2-methylpropyl N-[(2S)-1-oxidanylidene-1-[[(2S)-1-oxidanyl-3-[(3S)-2-oxidanylidenepyrrolidin-3-yl]propan-2-yl]amino]-3-phenyl-propan-2-yl]carbamate 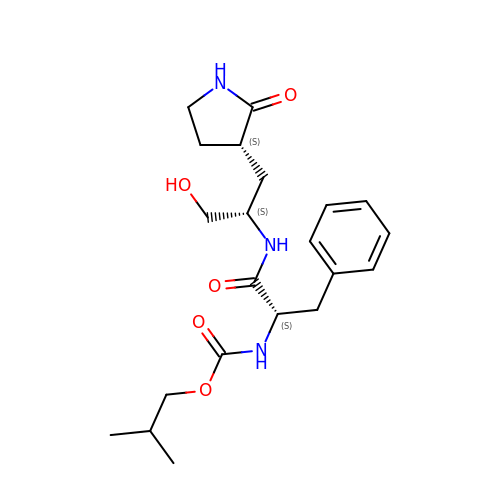| C21 H31 N3 O5 | OETPXUIOYJZSTO-BZSNNMDCSA-N> CHREPPPETPDINQLPPSILLKIFSNLSLDERCLSASLVCKYWRDLCLDFQFWKQLDLSSRQQVTDELLEKIASRSQNIIEINISDCRSMSDNGVCVLAFKCPGLLRYTAYRCKQLSDTSIIAVASHCPLLQKVHVGNQDKLTDEGLKQLGSKCRELKDIHFGQCYKISDEGMIVIAKGCLKLQRIYMQENKLVTDQSVKAFAEHCPELQYVGFMGCSVTSKGVIHLTKLRNLSSLDLRHITELDNETVMEIVKRCKNLSSLNLCLNW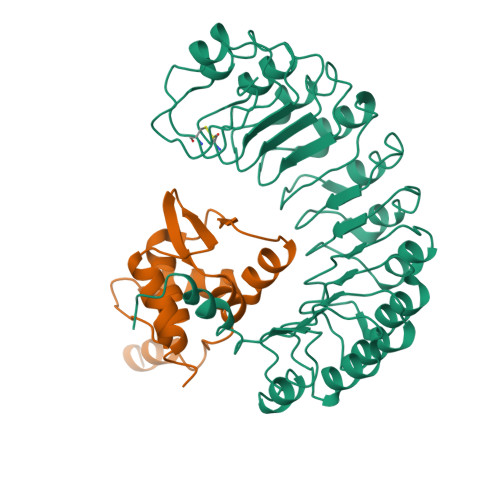IINDRCVEVIAKEGQNLKELYLVSCKITDYALIAIGRYSMTIETVDVGWCKEITDQGATLIAQSSKSLRYLGLMRCDKVNEVTVEQLVQQYPHITFSTVLQDCKRTLERAYQMGWTPNMSAASS;> SVFAYESSVHSTNVLLSLNDQRKKDVLCDVTIFVEGQRFRAHRSVLAACSSYFHSRIVGQADGELNITLPEEVTVKGFEPLIQFAYTAKLILSKENVDEVCKCVEFLSVHNIEESCFQFLKFKFLD> LRRSAVRYLKARPKTVNIEPGSNRFLDPNVEAKAKDIFAVPEFPNKAVLHNWRFFIKAGKAATGPPVG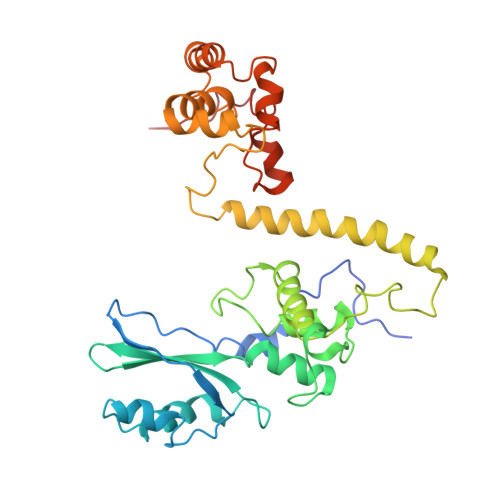QEFSKLGLKAMDFAKAFNDRTKPHFKDDIELIVRIQVYFDKSYIFRIEPPPTAWFLLRAIRKKRGETGPVVLRGNYCAYLTLEMCYEIAKMKQMSWGKVEYPPIEVRVRRVVGQARRMGIAIIGIDTVHSSPVKGMTEKQYLEESEKHRKVHMIQYEALKAKELESAPLIERLHRPNMAPLTNTQLEEGLKDANLLNALWKSSHPKSLFTQDTRDREMARRYLNTRGWFKEMTPEEMRVVFLNYRLPKQEDHQRQLNMTNGQAQSQAYWSRDAASPQ>[2x]AQYEDGKQYTTLEKPVAGAPQVLEFFSFFCAHAYQFEEVLHISDNVKKKLPEGVKM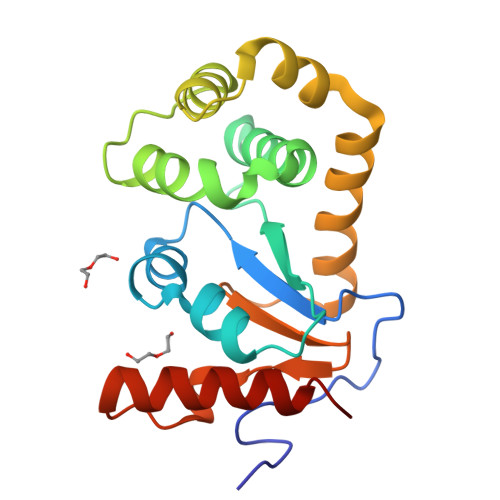TKYHVNFMGGDLGKDLTQAWAVAMALGVEDKVTVPLFEGVQKTQTIRSASDIRDVFINAGIKGEEYDAAWNSFVVKSLVAQQEKAAADVQLRGVPAMFVNGKYQLNPQGMDTSNMDVFVQQYADTVKYLSEKK> GMPENTAMAALLPE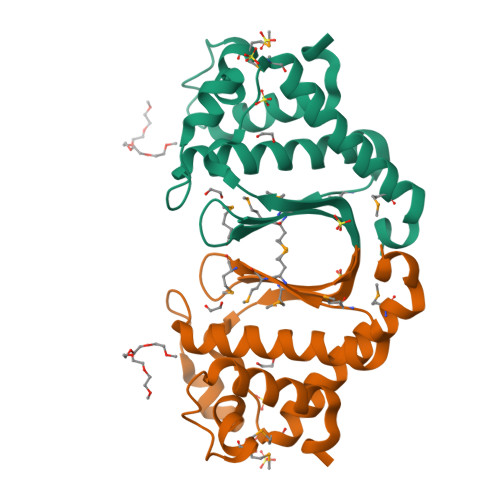ESLFFRELVKQWRAQDSYGTWEKKSDMELLAPYVLDKEQRRAIPIIGDPDPEILWRVELFYNAVGLATERASGVMVSPMMKMSHEGFGRMVLIAGRLIVVNKQLRDVHRFGFPSMEKLAEEGDKLVAGALEMIEKFPEVARF> MKYFTVFTALTALFAQASASAIPAVRSTLTPRQNTTASCANSATSRSCWGEYSIDTNWYDVTPTGVTREYWLSVENSTITPDGYTRSAMTFNGTVPGPAIIADWGDNLIIHVTNNLEHNGTSIHWHGIRQLGSLEYDGVPGVTQCPIAPGDTLTYKFQVTQYGTTWYHSHFSLQYGDGLFGPLIINGPATADYDEDVGVIFLQDWAHESVFEIWDTARLGAPPALENTLMNGTNTFDCSASTDPNCVGGGKKFELTFVEGTKYRLRLINVGIDSHFEFAIDNHTLTVIANDLVPIVPYTTDTLLIGIGQRYDVIVEANAAADNYWIRGNWGTTCSTNNEAANATGILRYDSSSIANPTSVGTTPRGTCEDEPVASLVPHLALDVGGYSLVDEQVSSAFTNYFTWTINSSSLLLDWSSPTTLKIFNNETIFPTEYNVVALEQTNANEEWVVYVIEDLTGFGIWHPIHLHGHDFFIVAQETDVFNSDESPAKFNLVNPPRRDVAALPGNGYLAIAFKLDNPGSWLLHCHIAWHASEGLAMQFVESQSSIAVKMTDTAIFEDTCANWNAYTPTQLFAEDDSGI

Laccases (EC 1.10.3.2; benzenediol:oxygen oxidoreductases) belong to the class of multicopper oxidases catalyzing the oxidation of phenols accompanied by the reduction of molecular oxygen to water. Laccases are composed of two or three structurally similar cupredoxin-like domains. The active site of laccases comprises four Cu atoms classified into three types depending on their spectroscopic characteristics. Type 2 and type 3 copper ions form a T2/T3 cluster responsible for the reduction of molecular oxygen to water.

The aim of the study presented here is to determine the structure of B. aclada laccase containing the complete set of copper ions. For this purpose, crystals of the type 2 copper-depleted form of B. aclada laccase were soaked in solutions containing Cu+ or Cu2+ ions. Restoration of the native form of the enzyme was only observed in the experiment employing Cu+ ions. The structure of T2D+Cu+ was solved at 2.3 Å resolution. Superimposition of the T2D+Cu+ and T2D structures using the coordinates of 525 equivalent Cα atoms gave an r.m.s.d. of 0.16 Å. Residues 1–14 (the numbering given is according to the T2D structure) and residues 405–408 were not located in the electron-density map for T2D+Cu+. It should be noted that in the structure of T2D Cu2 is completely absent and the sum of occupancies of the copper ions in T2D (2.6) is almost equal to the content of copper ions per molecule for the enzyme in solution as determined by mass spectrometry. In the T2D+Cu+ structure the type 2 copper ion has a square-planar coordination formed by the His87 N∊ and His429 N∊ atoms and the O atom of a water molecule. In the T2D structure His429 is coordinated to Cu3α by the Nδ atom. Thus, the removal of type 2 copper ions could be associated with changes in the orientation of the side chain of His429.>RLHIQNGHFVLNGQRVFLSGGNLPWMSYAYDFGDGQWQRNKNRIEPEFKKLHDAGGNSMRLWIHIQGETTPAFNDQGFVTGPDKQGTMLDDMKDLLDTAKKYNILVFPCLWNAAVNQDSHNRLDGLIKDQHKLQSYIDKALKPIVNHVKGHVALGGWDLM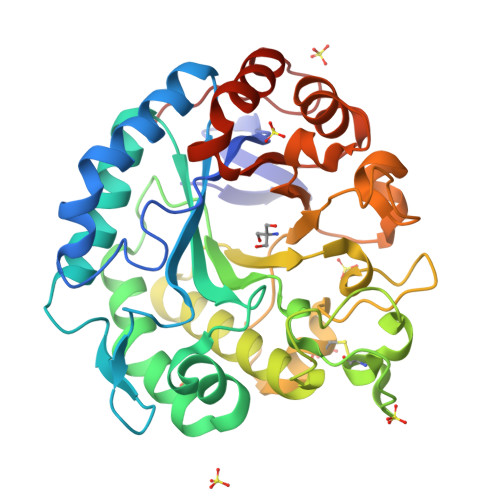NEPEGMMIPDKHNAEKCYDTTALKNSGAGWAGNKYLYQDILRFLNWQADAIKTTDPGALVTMGVWNPKSNTDHFNMNNHYSDHCLRLAGGKQKGVFDFYQFHSYSWQGKWDEVAPFTHQASDYGLHKPIVVGEFWEQDGGGMTITQMFNYVYNHGYAGAWSWHLVQRGDNQRKGITNIKDKTSNGKIPISL[2x]>XTTLSDKDKSTVKALWGKISKSADAIGADALGRMLAVYPQTKTYFSHWPDMSPGSGPVKAHGKKVMGGVALAVSKIDDLTTGLGDLSELHAFKMRVDPSNFKILSHCILVVVAKMFPKEFTPDAHVSLDKFLASVALALAERYR[2x];>[2x]VEWTQQERSIIAGIFANLNYEDIGPKALARCLIVYPWTQRYFGAYGDLSTPDAIKGNAKIAAHGVKVLHGLDRAVKNMDNINEAYSELSVLHSDKLHVDPDNFRILGDCLTV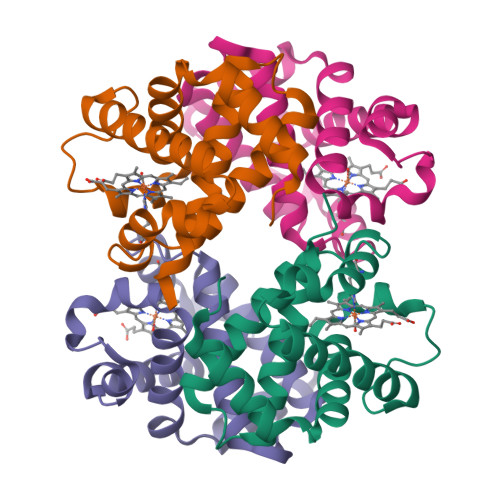VIAANLGDAFTVETQCAFQKFLAVVVFALGRKYH> MEILRYLMDPDTFTSNFNNGIGRHKTYLCYEVERLDNGTSVKMDQHMGFLCNESGRHAALRFLDLVPSLQLDPAQIYRVTWFISWSPCFSWGCAGEVRAFLQENTHVRLRIKAARIYDYDPLYKEALQMLRDAGAQVSIMTYDEFE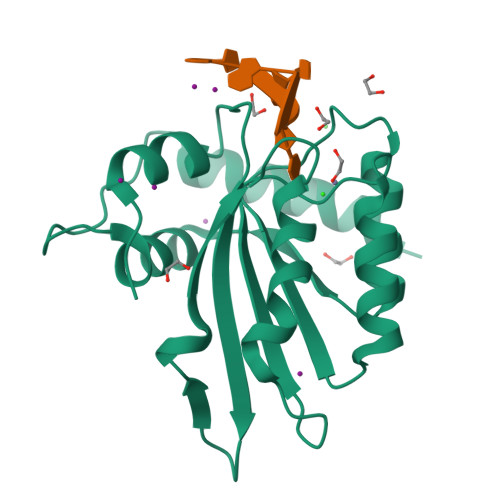YCWDTFVYRQGCPFQPWDGLEEHSQALSGRLRAILQLEHHHHHH> MNNDHINLKVAGQDGSVVQFKIKRHTPLSKLMKAYCERQGLSMRQIRFRFDGQP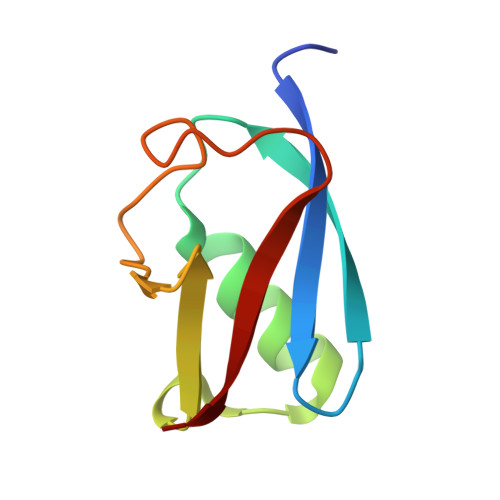INETDTPAQLEMEDEDTIDVFQQ>[2x]DDFAKLEEQFDAKLGIFALDTGTNRTVAYRPDERFAFASTIKALTVGVLLQQKSIEDLNQRITYTRDDLVNYNPITEKHVDTGMTLKELADASLRYSDNAAQNLILKQIGGPESLKKELRKIGDEVTNPERFAPELNEVNPGETQDTSTARALVTSLRAFALEDKLPSEKRELLIDWMKRNTTGDALIRAG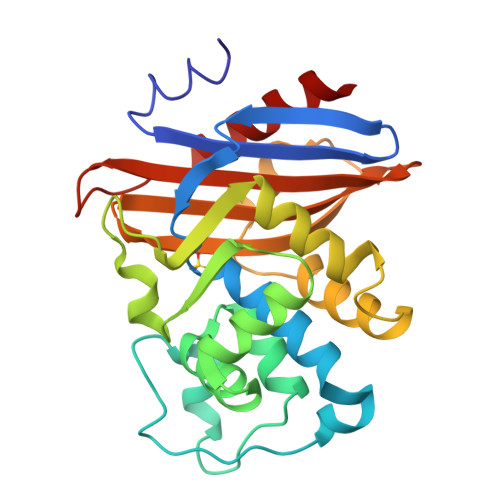VPDGWEVADKTGAASYGTRNDIAIIWPPKGDPVVLAVLSSRDKKDAKYDDKLIAEATKVVMKALN> SMSLQETRKAKSSSPKKQNDVRVKFEHRGEKR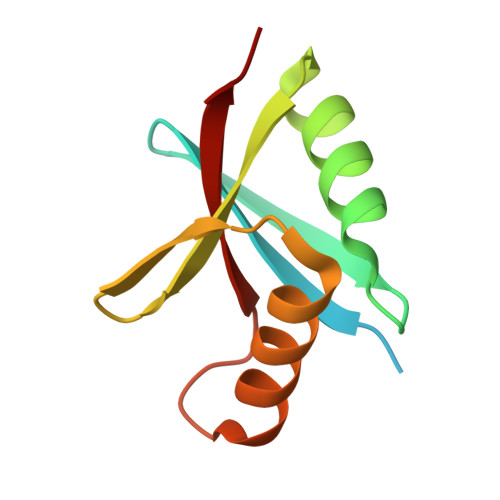ILQFPRPVKLEDLRSKAKIAFGQSMDLHYTNNELVIPLTTQDDLDKAVELLDRSIHMKSLKILLVING> MAHHHHHHSAALEVLFQGPGYSSGPELDNRVIFQSFSLYQPYESNMYKILATKGDLLKEWGITDVWLPPAYRSFNMARYMEGYAIADRYDLGEFNQGPNNERATKYGTSDELKDMIDKLHAAGLKVQLDLVPNQLLGLNGREAVYVTRVDNNGDLFKNPYTTGLTTRIRADLYLAYTKGGGQGQAKYGYIKEWNKNYFNGTSLQGQGMGRVMTDDNGKPYRFFGPNDPRNYLPSWLEEAAAANKINTV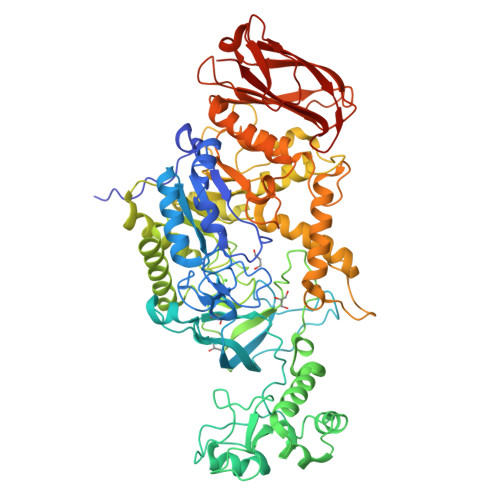DTYLPVDGWYAAKDAATSDQYWKPMLIHYAKDKGYLSFMSQHGFATVDDIINGDNAEIAKWTNAYIQSRPEYGFGSEERSYKNDNTGVDDQDQFLFVEENGSTKHNIHNTIHGNYEFLVGLDIDNSNPTVRKEQIHWMNWLLDTYKFDGFRIDAATHFDKQVLLDEADVRKAHFGNDLNNHLSYIESYTSKAEKFENENGNPHLTMDWALYYTLQDTLGKGTPSQKLSTIATNSVVNRSGSGSAHAIPNWSFVNNHDQEKNRVNTIMLDLYGIKTGEKYTTTPPKSFADLYDKETEKKALAIYKDDMKRVDKKYAPNNVVSQYAFLLTNKDTVPTIYYGDLYQTDASYMSKPTLYYEPITKLLKMRKAYAYGGQKITGYTSNTSPETAGQDLIASVRYGKDRYTGVAVVIGTNPKTDTTIKVDMGTKHANQVFKDATGFHSEKLVADNKGVLTIRVKGTANALVKGYLGVWVPTKDKA> HHHHHHSSGENLYFQGHMAPIQDPVAFIKQMPYHQVVKELALSRCLAQVSDSDKAFSLDAARTANAMREWMPFDIESGDEKINVLIDKYKSRINEFHSETKDKSQGVTLNCLRLYHSPELDKLSRQLIAGNPDRTWNQDNAK

The S. marcescens Rap proteins represent founder members of a new bacterial protein family, members of which represent immunity proteins for T6-secreted toxins, as exemplified by Rap1a and Rap2a. We have determined the structures of two members of this family, Rap1b and Rap2b, revealing a new protein fold. The Rap subunit is constructed around a helical bundle of five helices (α2–α6). The Rap proteins display an extensive dimerization interface, consistent with the observation that each Rap protein exists as a stable dimer in solution.

Well-ordered crystals of Rap1b and Rap2b were obtained and the structures were elucidated at 1.9 Å and 2.0 Å resolution respectively. The asymmetric unit of the Rap1b structure consists of a single subunit and crystallographic symmetry generates the dimer. An overlay of Rap1b and Rap2b subunits matches 71 Cα atoms with a r.m.s.d. of 1.4 Å. A disulphide linkage (Cys54–Cys120 in Rap1b, Cys41–Cys101 in Rap2b) tethers α2 and α5 together. By virtue of being longer than Rap2b, Rap1b has an extension of five residues at the N-terminus and 13 at the C-terminus, the latter of which form a short helix α7. These segments of Rap1b are on the surface of the molecules at opposite ends of the dimer. The Rap1b dimer uses almost 24% of the accessible surface area of a subunit in formation of the dimer. Surprisingly for proteins with such low pI values, the striking surface feature conserved in Rap1b and Rap2b structures is a crescent-shaped basic patch on either side of the dimer. However, the role of Rap1b and Rap2b is not yet known. While they do not appear to play a role in self-resistance, they may play a role in resistance towards closely related bacteria secreting similar toxins.> ADYQVYAWGINDPTEGERTVIKDPWDSVAS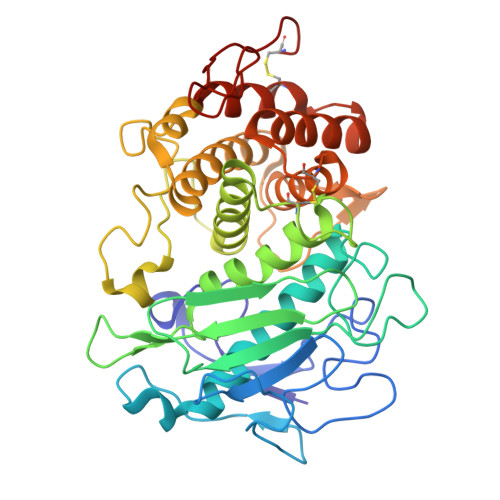EFTWISDGSTNYTTSRGNNGIAQSNPSGGPSYLNNYRPSSSSLSFKYPYSVSSSPPSSYIDASIIQLFYTANIYHDLLYTLGFTEKAGNFEYNTNGQGGLGNDYVILNAQDGSGTNNANFATPPDGQPGRMRMYVWTESTPYRDGSFEAGIVIHEYTHGLSNRLTGGPANSNCLNALESGGMGEGWSDFMATAIRLKPGDKRSTDYTMGEWASNRAGGIRQYPYSTSLSTNPLTYTSVNSLNAVHAIGTVWASMLYEVLWNLIDKHGKNDAPKPTLRDGVPTDGKYLAMKLVMDGMALQPCNPNFVQARDAILDADTALTGGENQCEIWTAFAKRGLGAGAKYSSRNRVGSTEVPSGVC>VEHISKGNNCLDAAKACNLDDTCKKYRSAYITPCTTSMSNEVCNRRKCHKALRQFFDKVPAKHSYGMLFCSCRDIACTERRRQTIVPVCSYEERERPNCLSLQDSCKTNYICRSRLADFFTNCQPESRSVSNCLKENYADCLLAYSGLIGTVMTPNYVDSSSLSVAPWCDCSNSGNDLEDCLKFLNFFKDNTCLKNAIQAFGNGSDVTMWQPAPPVQTTTATTTTAFRVKNKPLGPAGSENEIPTHVLPPCANLQAQKLKSNVSGSTHLCLSDSDFGKDGL[2x];>SPDKQMA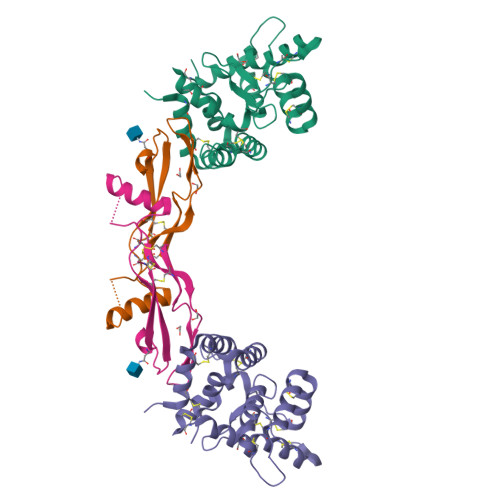VLPRRERNRQAAAANPENSRGKGRRGQRGKNRGCVLTAIHLNVTDLGLGYETKEELIFRYCSGSCDAAETTYDKILKNLSRNRRLVSDKVGQACCRPIAFDDDLSFLDDNLVYHILRKHSAKRCGCI[2x]> MDISQH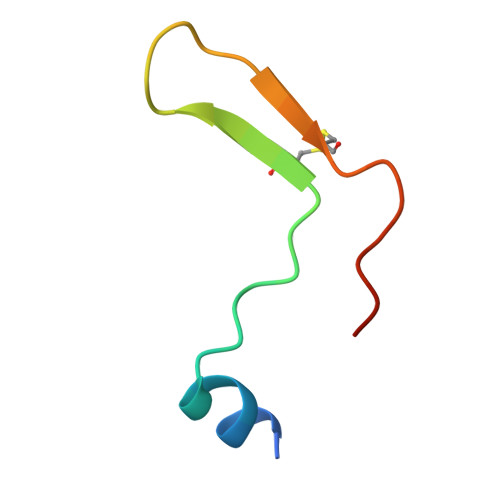ATDIGMGPATSCYTSTIPPPKQVCIQQAVKATL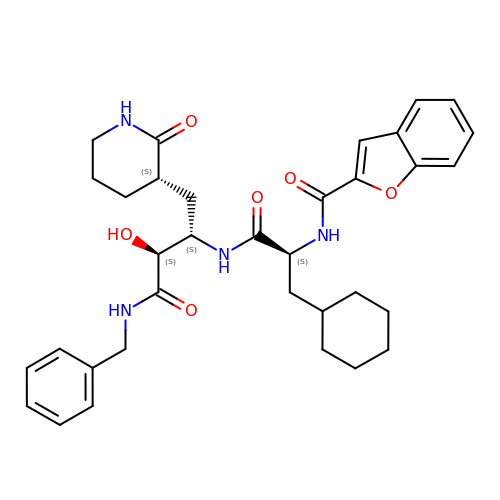N-[(2S)-3-cyclohexyl-1-oxidanylidene-1-[[(2S,3S)-3-oxidanyl-4-oxidanylidene-1-[(3S)-2-oxidanylidenepiperidin-3-yl]-4-[(phenylmethyl)amino]butan-2-yl]amino]propan-2-yl]-1-benzofuran-2-carboxamide | C34 H42 N4 O6 | QBWBVQMSMXVSSF-YRUYCOJQSA-N>MTSHFMLRRALLPLAIAALAGCSLAPTYERPQAPVASHWQAADAEGARAQALDWQTFIVDADLRRAVDTALSNNRSLRQALLDIEAARAQYRIQRADRLPSINANASGNRQRLPADLSQTGRSEVTSNYQVGLGLAEYEVDLFGRVRNLSEAALETYLATEEATRATQISLVAEVIQAYLTRDGALRRMALVEQTLDSRMASLELVSQRRAAGAATALDYQEAVGLAEQARAERESTERQLRQADNALVLLLGTPDAARLLPATPRDDLMVLQDIAPGTSSELIERRPDILASEHRLKARNADIGAARAAFFPRISLTGSVGSSSAELSGLFDGGSRAWSFAPTLSLPIFAGGRNRANLDLAEVRQDAAVADYEGTIQTAFREVADALAATDTLRREEAARQALAGSSEAAMALAKARYEGGVDDYLRYLDAQRSTFSNQTTLIQISTERQIALVDLFRSLGGGWGQTEPMAGIGAEHHHHHH[3x];>MNKFREWITFSVISCLVAVTLVGCDKPEEQREEAPAREVDVLSVKTEPFTVFAELPGRIEPVRVAEVRARVAGIVLKRTFEEGADVKAGDVLFQIDPAPFKAALSRAQGELARAEAQLFQAQAMVRRYEPLVKIDAVSQQDFDNAMAALQSAQADKRSAQANVETARLDLGYAEVRAPIAGRIGRAQVTEGALVGQGEATLLARIQQLDPVYADFTQPAADALRLRAAIAEGKVAGASDQPLSLRVDGTDIERKGTLLFTDISVDRSTGQIALRGQ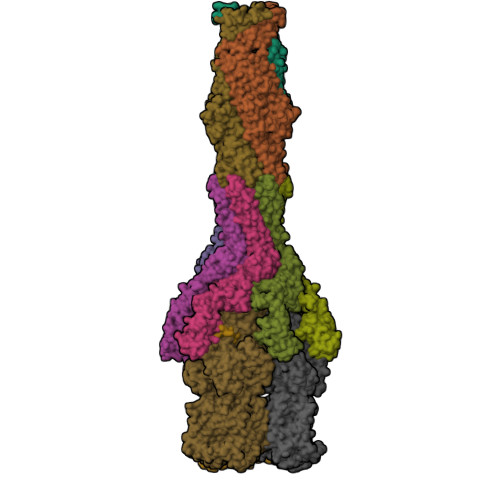FDNPEGVLLPGMYVRVRTPQGLNQNAILVPQRAVQRSADGQASVMLLGEGDTVEVRQVTTGAMQGSRWQISEGLQAGDKVITSSLAAIRPGAKVIPREQGAAEKAPQSQAQWSHPQFEK[6x];>[3x]MPLFFIRRPNFAWVVALFISLGGLLVIPFLPVAQYPNVAPPQITVTATYPGASAQVLTDSVTSVIEEELNGAKNLLYFESTSNANGIAEITVTFQPGTDPELAQVDVQNRLKKAEARMPQAVLTLGIQTEQATAGFLLIYSLRYKDGDKNANTTALADYAVRNVNNEIRRLPGVGKLQFFDSEAAMRVWIDPQKLVGYGLSIDDVNNAIRTQNVQVPAGAFGSTPGSSEQELTATLTVKGTLDNPEEFAAIVLRANQDGSRLTLGDVARIEVGSQDYNFGSRQDGKPAVAAAVQLSPGANAIQTAEAVKQRLTELSANFPDNVEFSVPYDTSRFVDVAIDKVIMTLIEAMVLVFLVMFLFLQNVRYTLIPSIVVPVCLLGTLTFMYLLGFSVNMMTMFGMVLAIGILVDDAIVVVENVERIMAEEGLAPVPATIKAMGQVSGAIIGITLVLSAVFLPLAFMAGSVGVIYQQFSLSLAVSILFSGFLALTFTPALCATLLKPIPVGHHEKTGFFGWFNRKFTSLTSRYTKLNDKLVPRAGRVMFIYLGVVVLMGFLYMRLPESFVPVEDQGYMIVDIQLPPGATRERTSAAGGELESFLMAREAVQTTFLVLGFSFSGMGENAAIAFPLLKDWSERDSSQSPEAESAAVNQHFANLDDGAIMAVPPPPVEGLGNSGGFALRLQDRAGLGRDALLAARDEVLGKVNGNPKFLYAMMEGLAEAPQLRLVIDREQARTLGVSFEAISSALSTAFGSSVINDFANAGRQQRVVVQAEQAERMTPESVLRLHVPNDSGSLVPLSAFVTTSWEEGPVQVARYNGYPSIRIAGDAAPGVSTGEAMLELERIAAELPEGIGYEWTGLSYQERVASGQATMLFALAITVVFLLLVALYESWAIPLTVMLIVPVGALGAVLAVTAIGLPNDVYFKVGLITVIGLAAKNAILIVEFAKDLWEDGYSLRDAAVEAARLRFRPIIMTSMAFMLGVVPLAIATGAGAASQRALGTGVLGGMLSATMLGVIFVPIFFVWVLSLLRTKPQQTDNHPLHKAE>VRSSSRTPSDKPVAHVVANPQ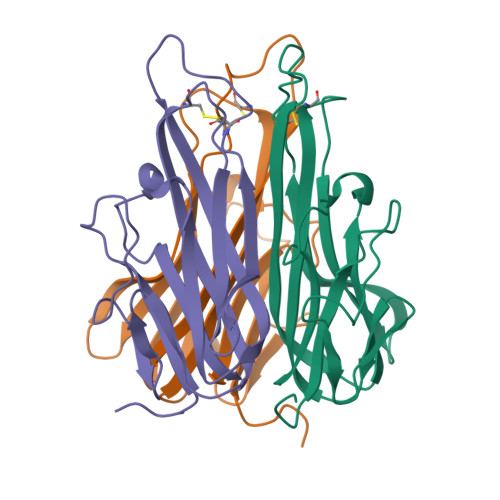AEGQLQWLNDRANALLANGVELRDNQLVVPSEGLYLIYSQVLFKGQGCPSTHVLLTHTISRIAVSYQTKVNLLSAIKSPCQRETPEGAEAKPWYEPIYLGGVFQLEKGDRLSAEINRPDYLDFAESGQVYFGIIAL[3x]methyl 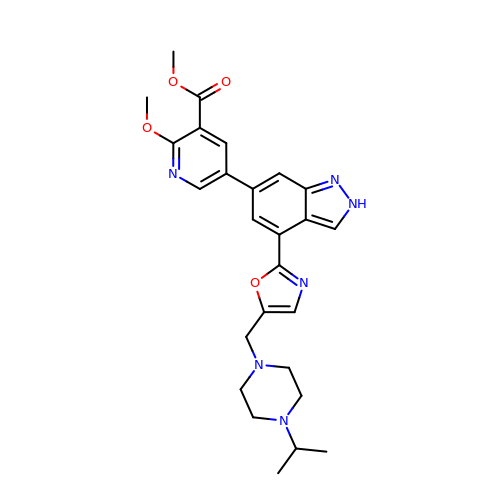2-methoxy-5-[4-[5-[(4-propan-2-ylpiperazin-1-yl)methyl]-1,3-oxazol-2-yl]-2~{H}-indazol-6-yl]pyridine-3-carboxylate | C26 H30 N6 O4 | RKURWVGLSOZAMD-UHFFFAOYSA-N> HHHHHHSSGVPRGSHMRILVIAGCSEGFVMPLVPLSWALRAAGHEVLVAASENMGPTVTGAGLPFAPTCPSLDMPEVLSWDREGNRTTMPREEKPLLEHIGRGYGRLVLRMRDEALALAERWKPDLVLTETYSLTGPLVAATLGIPWIEQSIRLASPELIKSAGVGELAPELAELGLTDFPDPLLSIDVCPPSMEAQPKPGTTKMRYVPYNGRNDQVPSWVFEE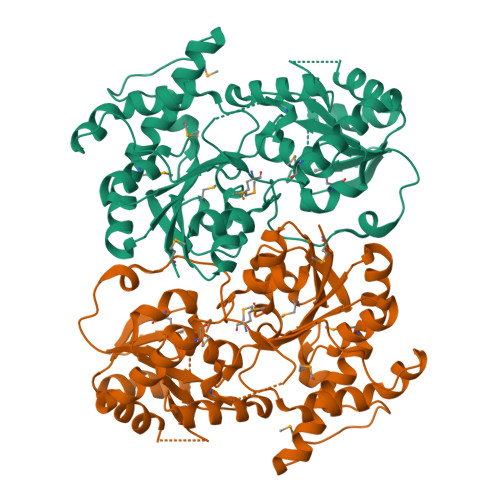RKQPRLCLTFGTRVPLPNTNTIPGGLSLLQALSQELPKLGFEVVVAVSDKLAQTLQPLPEGVLAAGQFPLSAIMPACDVVVHHGGHGTTLTCLSEGVPQVSVPVIAEVWDSARLLHAAGAGVEVPWEQAGVESVLAACARIRDDSSYVGNARRLAAEMATLPTPADIVRLIEQA stemmadenine acetate | C23 H29 N2 O4 | 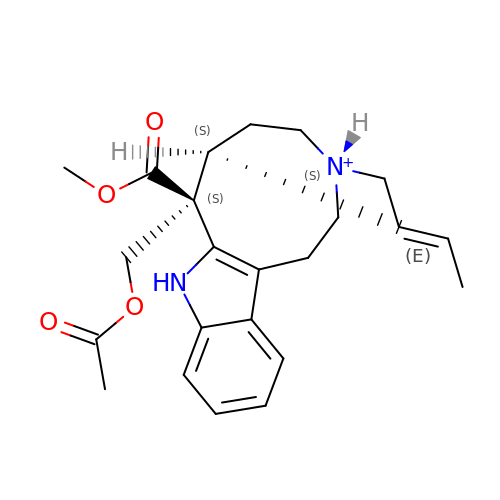ZNCUMLJVNWXVLT-ISNKGDJGSA-O>[4x]MYTNSDFVVIKALEDGVNVIGLTRGADTRFHHSEKLDKGEVLIAQFTEHTSAIKVRGKAYI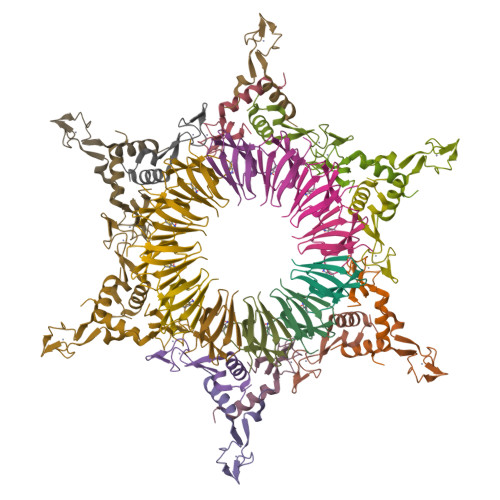QTRHGVIESEGKK;>[6x]MVIATDDLEVACPKCERAGEIEGTPCPACSGKGVILTAQGYTLLDFIQKHLNK> MKTLVHVASVEKGRSYEDFQKVYNAIALKLREDDEYDNYIGYGPVLVRLAWHISGTWDKHDNTGGSYGGTYRFKKEFNDPSNA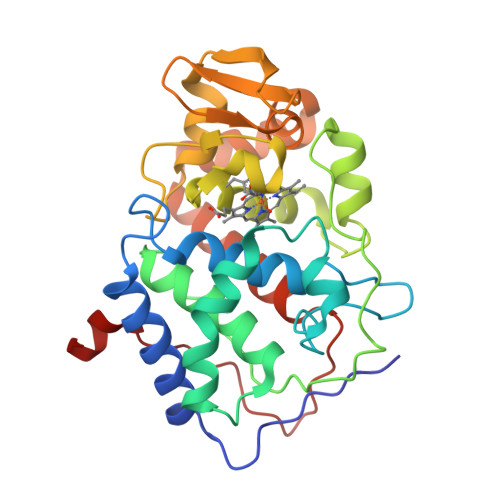GLQNGFKFLEPIHKEFPWISSGDLFSLGGVTAVQEMQGPKIPWRCGRVDTPEDTTPDNGRLPDMDKDAGYVRTFFQRLNMNDREVVALMGAHALGKTHLKNSGYEGPWGAANNVFTNEFYLNLLNEDWKLEKNDANNEQWDSKSGYMMLPTDYSLIQDPKYLSIVKEYANDQDKFFKDFSKAFEKLLENGITFPKDAPSPFIFKTLEEQGL>MEKKMSGSRPTQSSEGSRRSRHSARIIAQTTVDAKLHADFEESGSSFDYSTSVRVTGPVVENQPPRSDKVTTTYLHHIQKGKLIQPFGCLLALDEKTFKVIAYSENASELLTMASHAVPSVGEHPVLGIGTDIRSLFTAPSASALQKA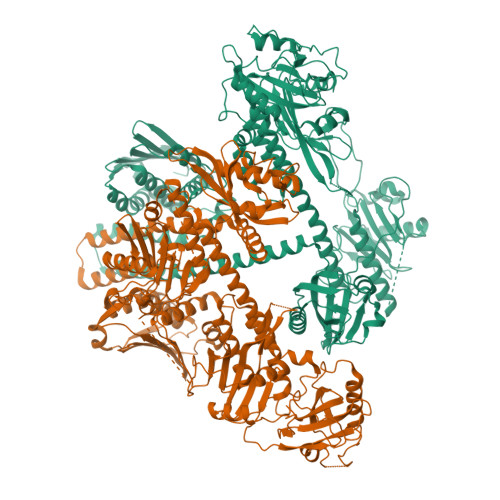LGFGDVSLLNPILVHCRTSAKPFYAIIHRVTGSIIIDFEPVKPYEVPMTAAGALQSYKLAAKAITRLQSLPSGSMERLCDTMVQEVFELTGYDRVMAYKFHEDDHGEVVSEVTKPGLEPYLGLHYPATDIPQAARFLFMKNKVRMIVDCNAKHARVLQDEKLSFDLTLCGSTLRAPHSCHLQYMANMDSIASLVMAVVVNEEDGEGDAPDATTQPQKRKRLWGLVVCHNTTPRFVPFPLRYACEFLAQVFAIHVNKEVELDNQMVEKNILRTQTLLCDMLMRDAPLGIVSQSPNIMDLVKCDGAALLYKDKIWKLGTTPSEFHLQEIASWLCEYHMDSTGLSTDSLHDAGFPRALSLGDSVCGMAAVRISSKDMIFWFRSHTAGEVRWGGAKHDPDDRDDARRMHPRSSFKAFLEVVKTRSLPWKDYEMDAIHSLQLILRNAFKDSETTDVNTKVIYSKLNDLKIDGIQELEAVTSEMVRLIETATVPILAVDSDGLVNGWNTKIAELTGLSVDEAIGKHFLTLVEDSSVEIVKRMLENALEGTEEQNVQFEIKTHLSRADAGPISLVVNACASRDLHENVVGVCFVAHDLTGQKTVMDKFTRIEGDYKAIIQNPNPLIPPIFGTDEFGWCTEWNPAMSKLTGLKREEVIDKMLLGEVFGTQKSCCRLKNQEAFVNLGIVLNNAVTSQDPEKVSFAFFTRGGKYVECLLCVSKKLDREGVVTGVFCFLQLASHELQQALHVQRLAERTAVKRLKALAYIKRQIRNPLSGIMFTRKMIEGTELGPEQRRILQTSALCQKQLSKILDDSDLESIIEGCLDLEMKEFTLNEVLTASTSQVMMKSNGKSVRITNETGEEVMSDTLYGDSIRLQQVLADFMLMAVNFTPSGGQLTVSASLRKDQLGRSVHLANLEIRLTHTGAGIPEFLLNQMFGTEEDVSEEGLSLMVSRKLVKLMNGDVQYLRQAGKSSFIITAELAAANK[2x]2-[(3S)-3-AMINOPIPERIDIN-1-YL]-1-(2-CYANOBENZYL)-5-METHYL-4,6-DIOXO-3,4,5,6-TETRAHYDROPYRROLO[3,4-D]IMIDAZOL-1-IUM 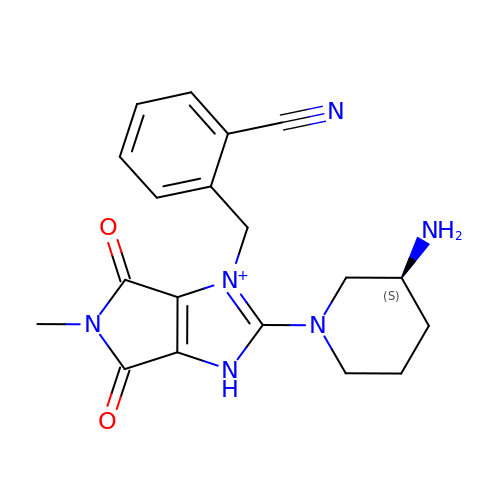| C19 H21 N6 O2 | WVRGIUWTFUXDGX-AWEZNQCLSA-O> MPKRTDIKSILILGAGPIVIGQACEFDYSGAQACKALREEGYRVINVNSNPATIMTDPEMADATYIEPIHWEVVRKIIEKERPDAVLPTMGGQTALNCALELERQGVLEEFGVTMIGATADAIDKAEDRRRFDVAMKKIGLETARSGIAHTMEEALAVAADVGFPCIIRPSFTMGGSGGGIAYNREEFEEICARGLDLSPTKELLIDESLIGWKEYEMEVVRDKNDNCIIVCSIENFDAMGIHTGDSITVAPAQTLTDKEYQIMRNASMAVLREIGVETGGSNVQFAVNPKNGRLIVIEMNPRVSRSSALASKATGFPIAKVAAKLAVGYTLDELMNDITGGRTPASFEPSIDYVVTKIPRFNFEKFAGANDRLTTQMKSVGEVMAIGRTQQESLQKALRGLEVGATGFDPKVSLDDPEALTKIRRELKDAGADRIWYIADAFRAGLSVDGVFNLTNIDRWFLVQIEELVRLEEKVAEVGITGLNADFLRQLKRKGFADARLAKLAGVREAEIRKLRDQYDLHPVYKRVDTCAAEFATDTAYMYSTYEEECEANPSTDREKIMVLGGGPNRIGQGIEFDYCCVHASLALREDGYETIMVNCNPETVSTDYDTSDRLYFEPVTLEDVLEIVRIEKPKGVIVQYGGQTPLKLARALEAAGVPVIGTSPDAIDRAEDRERFQHAVERLKLKQPANATVTAIEMAVEKAKEIGYPLVVRASYVLGGRAMEIVYDEADLRRYFQTAVSVSNDAPVLLDHFLDDAVEVDVDAICDGEMVLIGGIMEHIEQAGVHSGDSACSLPAYTLSQEIQDVMRQQVQKLAFELQVRGLMNVQFAVKNNEVYLIEVNPRAARTVPFVSKATGVPLAKVAARVMAGKSLAEQGVTKEVIPPYYSV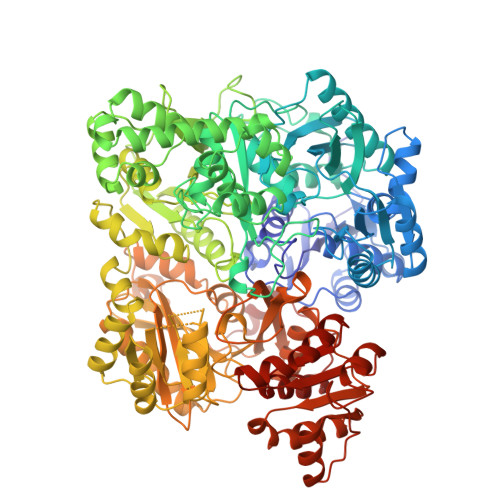KEVVLPFNKFPGVDPLLGPEMRSTGEVMGVGRTFAEAFAKAQLGSNSTMKKHGRALLSVREGDKERVVDLAAKLLKQGFELDATHGTAIVLGEAGINPRLVNKVHEGRPHIQDRIKNGEYTYIINTTSGRRAIEDSRVIRRSALQYKVHYDTTLNGGFATAMALNADATEKVISVQEMHAQIK4-[6-(benzylamino)imidazo[1,2-b]pyridazin-3-yl]benzonitrile 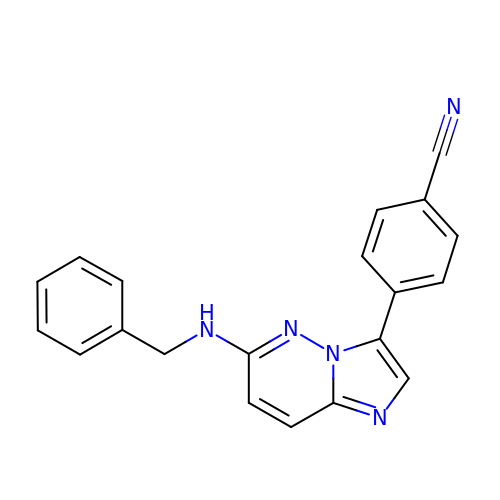| C20 H15 N5 | OXQTXNVWTNDAQF-UHFFFAOYSA-N>[3x]ASMRFTTEQIDYYGKACNASEDDLVV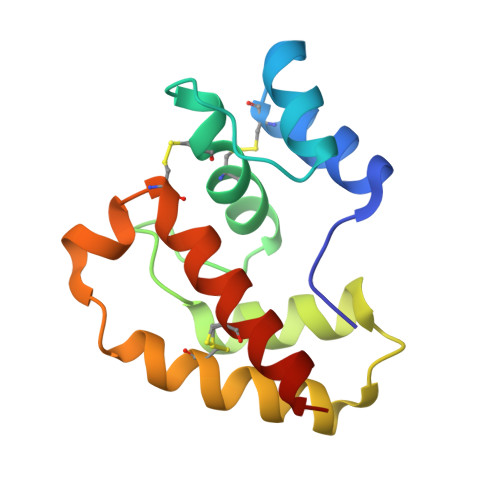VKSYKVPSTETGKCLMKCMITKLGLLNDDGSYNKTGMEAGLKKYWSEWSTEKIETINNKCYEEALLVSKEVVATCNYSYTVMACLNKQLDLDKST>[6x]DVYQEPTDPKFPQQWYLSGVTQRDLNVKAAWAQGYTGHGIVVSILDDGIEKNHPDLAGNY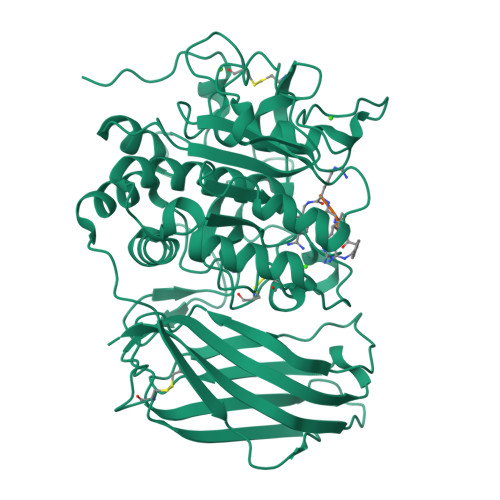DPGASFDVNDQDPDPQPRYTQMNDNRHGTRCAGEVAAVANNGVCGVGVAYNARIGGVRMLDGEVTDAVEARSLGLNPNHIHIYSASWGPEDDGKTVDGPARLAEEAFFRGVSQGRGGLGSIFVWASGNGGREHDSCNCDGYTNSIYTLSISSATQFGNVPWYSEACSSTLATTYSSGNQNEKQIVTTDLRQKCTESHTGTSASAPLAAGIIALTLEANKNLTWRDMQHLVVQTSKPAHLNANDWATNGVGRKVSHSYGYGLLDAGAMVALAQNWTTVAPQRKCIIDILTEPKDIGKRLEVRKTVTACLGEPNHITRLEHAQARLTLSYNRRGDLAIHLVSPMGTRSTLLAARPHDYSADGFNDWAFMTTHSWDEDPSGEWVLEIENTSEANNYGTLTKFTLVLYGTASGSLVPRGSHHHHHH> MHHHHHHMKSIDEQSLHNARRLFESGDIDRIEVGTTAGLQQIHRYLFGGLYDFAGQIREDNISKGGFRFANAMYLKEALVKIEQMPERTFEEIIAKYVEMNIAHPFLEGNG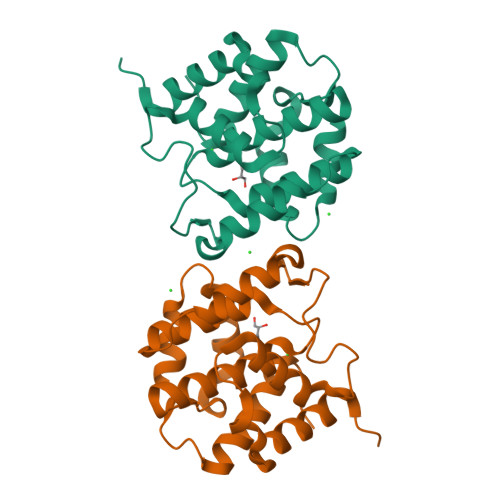RSTRIWLDLVLKKNLKKVVNWQNVSKTLYLQAMERSPVNDLRLRFLLKDNLTDDVDNREIIFKGIEQSYYYEGYEKG>NQPVNQPILAAAQSLHREATKWSSKGNDIIAAAKRMALLMAEMSRLVRGGSGTKRALIQCAKDIAKASDEVTRLAKEVAKQCTDKRIRTNLLQVCERIPTISTQLKILSTVKATMLGRTNISDEESEQATEMLVHNAQNLMQS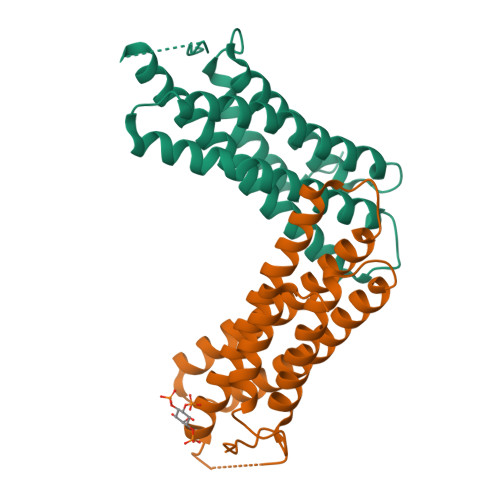VKETVREAEAASIKIRTDAGFTLRWVRKT[4x]> PAQDNSRFVIRDRNWHPKALTPDYKTSIARSPRQALVSIPQSISETTGPNFSHLGFGAHDHDLLLNFNNGGLPIGERIIVAGRVVDQYGKPVPNTLVEMWQANAGGRYRHKNDRYLAPLDP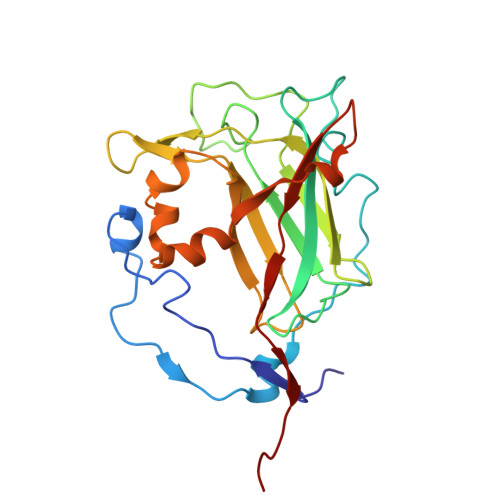NFGGVGRCLTDSDGYYSFRTIKPGPYPWRNGPNDWRPAHIYFGISGPSIATKLITQLYFEGDPLIPMCPIVKSIANPEAVQQLIAKLDMNNANPMDCLAYRFDIVLRGQRKTHFENC>[8x]MRGLSRRVQAMKPDAVVAVNAKALELRRQGVDLVALTAGEPDFDTPEHVKEAARRALAQGKTKYAPPAGIPELREALAEKFRRENGLSVTPEETIVTVGGSQALFNLFQAILDPGDEVIVLSPYWVSYPEMVRFAGGVVVEVETLPEEGFVPDPERVRRAITPRTKALVVNSPNNPTGAVYPKEVLEALARLAVEHDFYLVSDEIYEHLLYEGEHFS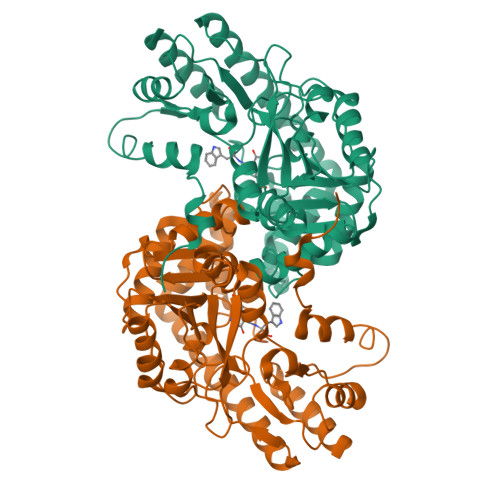PGRVAPEHTLTVNGAAKAFAMTGWRIGYACGPKEVIKAMASVSRQSTTSPDTIAQWATLEALTNQEASRAFVEMAREAYRRRRDLLLEGLTALGLKAVRPSGAFYVLMDTSPIAPDEVRAAERLLEAGVAVVPGTDFAAFGHVRLSYATSEENLRKALERFARVLGRA>MALAKRIDAALIMKDGRVVKGSNFENLRDSGDPVELGKFYSEIGIDELSFWDITASVEKRKTMLELVEKVAEQIDIPITVGGGIHDFETASELILRGADKVEFNTAAVENPSLITQIAQTFGSQAVVVYIAAKRVDGEFMVFTYSGTKNTGILLRDWVVEVEKRGAGEIVLGSIDRLGTKSGYDTEMIRFVRPLTTLPIIAHRGAGKMEHFLEAFLAGA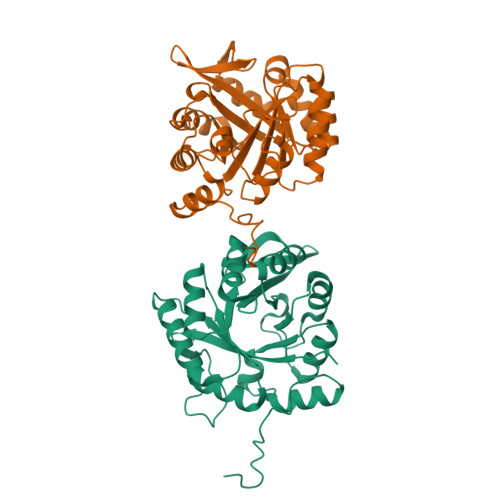DAAKADSVFHSREIDVRELKEYLKKHGVNVRLEGLGSLEHHHHHH[2x]>MEEIIVRGGNQLNGTVRIEGAKNAVLPILAASLLAEEGITTLDNVPILSDVFTMNQVIRHLNVDVDFDEQKNQVTIDASRQLEIEAPYEYVSQMRASIVVMGPLLARNGHAKVAMPG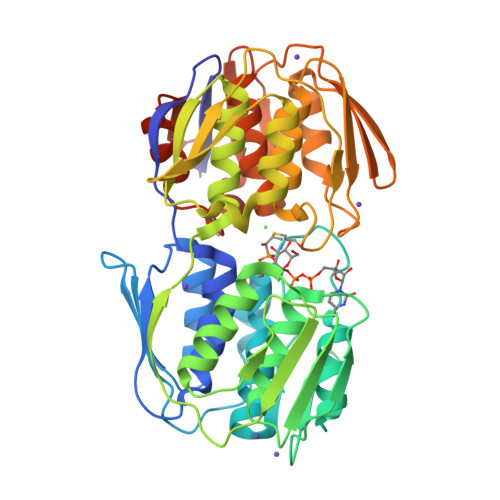GCAIGKRPIDLHLKGFQALGAKIIQKNGYIEAIADELIGNTIYLDFPSVGATQNIMMAAVKAKGTTIIENVAREPEIVDLANILNKMGAQVYGAGTETMRIEGVDHLHAVNHSIVQDRIEAGTFMVAAAMTQGNVLIADAISEHNRPLISKLIEMGAEIIEEEGGVRVIGPKHILPTDVKTMPHPGFPTDMQAQMTAIQLVAEGTSVVTETVFENRFQHLEEMRRMNAHVKIDGNVAIMDGNHELQGAEVYATDLRAAAALVLAGLKANGITRVRNLNYLDRGYYNFHIKLQQLGADVERVDMDQTSAEKTAQTIA[4x]>DHYNCVSSGGQCEYSACPIFTKIQGTCYRGKAKCCK[2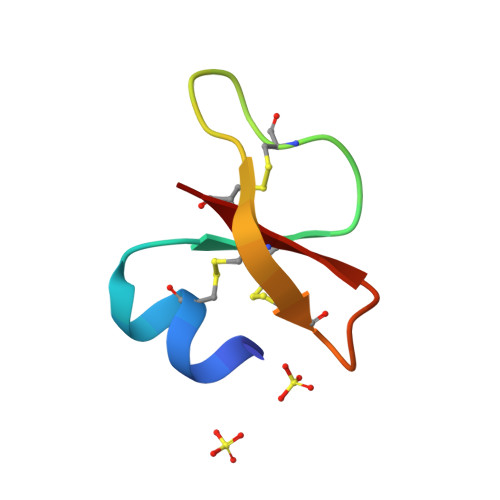x]Lectins are carbohydrate binding proteins unrelated to immunoglobulins that display no enzymatic activity towards the recognized sugars. Lectins purified from seeds of the Diocleinae subtribe exhibit a high degree of sequence identity notwithstanding that they show very distinct biological activities. In the present study, we used mass spectrometry to determine the amino acid sequence of a lectin from Canavalia boliviana seeds and solved its crystal structure in complex with Xman and the dimannosides Man(α1-3)Man(α1-O)Me and Man(α1-4)Man(α1-O)Me. Furthermore, we characterized the anti-inflammatory properties of Cbol, adding more data to the repertoire of wide biological activities displayed by this group of lectins, despite their highly identical sequence.

Originating from the crystallization condition, nine cadmium ions are observed in the structures Cbol:M13M and Cbol:M14M. Intriguingly, in all but one subunit of the dimannoside complexes, cadmium ions are found coordinated to two asparagines in the small helix Leu81-Val84. The carbohydrate electron densities of M13M and M14M and Xman complexes are well defined in all subunits. In the dimannoside complexes, none of the subunits are involved in extensive interactions with the symmetry mates around the carbohydrate-binding sites, a favourable feature that prevents bias in the structural analysis of the complexes. The O1-linked mannose of both dimannosides, M13M and M14M, as well as Xman, are bound to the monosaccharide binding site in an almost identical way to that observed for ConA, CGL and ConM. The O3- and O4-linked mannose (reducing mannoses, also called here the second mannose) are positioned in a previously described hydrophobic subsite, formed by Tyr12, Leu99 and Tyr100. The side chains of Tyr12, Leu99 and Tyr100 are opposite to the ring of the reducing mannose, which interacts with the protein mainly by hydrophobic and van der Waals interactions. Differences occur in the binding of the dimannosides as result of their distinct glycosidic linkage. Similarly to Cbol, the reducing mannose of M13M when in complex with ConA does not form hydrogen bonds with the protein. In the central cavity of Cbol in complex with dimannosides, there is a strong unexplained density in the vicinity of His127, Met129 and Asn131.

>[4x]ADTIVAVELDTYPNTDIGDPSYPHIGIDIKSVRSKKTAKWNMQNGKVGTAHIIYNSVGKRLSAVVSYPNGDSATVSYDVDLDNVLPEWVRVGLSATTGLYKETNTILSWSFTSKLKSNSTHETNALHFMFNQFSKDQKDLILQGDATTGRDGNLELTRVSSNGSPQGSSVGRALFYAPVHIWESSAVVASFDATFTFLIKSSDSHPADGIAFFISNIDSSIPSGSTGRLLGLFPDAN>[6x]MSNTADFRLQTSTLCHSFLLASANKQDTDYLTDLLDNTNIDLTCVPNGQEIIHS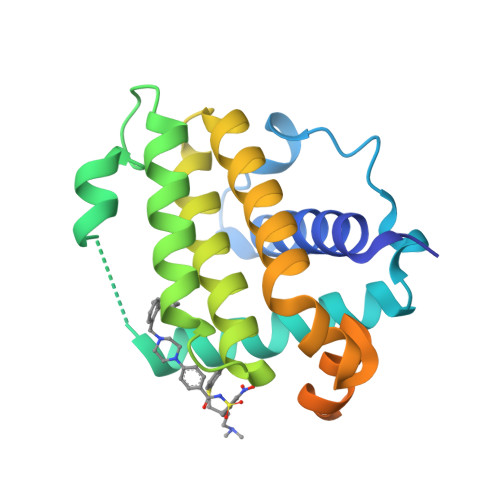LLQLVGDFNQRFSQTHEIEPVAQSLGIDSDKPVDKTALEIFYLEILNGLFEKLNWGRIVAMFAFLRILVLRLSKHGHSDAIQMLIKTTSQYSDEKLKNWINLHDGWSGLIEFSGRQFVNDGQELIWKTLRNVGGLATGAVGALGLAALVGYIANKI>[4x]MVTSPALRDVHVPHAYPEQQVDLGEITMNYAEAGDPDRPAVLLIPEQTGSWWSYEEAMGLLSEHFHVYAVDLRGQGRSSWTPKR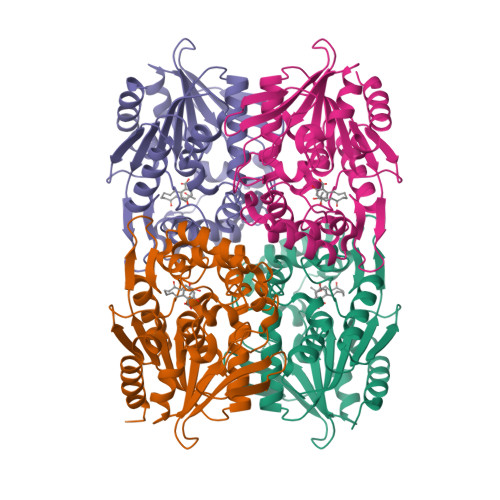YSLDNFGNDLVRFIALVVKRPVVVAGNSSGGVLAAWLSAYSMPGQLRGVLCEDPPFFASELVPAHGHSVRQGAGPVFELFRTYLGDQWSVGDWEGFCRAAGASASPMARSFVADGIPQHLQEYDPEWARVFYEGTVGLSCPHERMLGQVKTPVLLTHHMRGIDPETGNLLGALSDEQALRARRLMDSAGVTVDYESVPDASYMMHQSAPARYVEIFTRWAAALAPHHHHHH>MNKVHVSAVGTGLLKNSLSADNVKKEVEDLGLKDWDRLKFDDDRQNKIRDNFTTLKDLLLNFLKSKGKEASAELDSLLSAIEKLQHKKEELYVFLYTTNTWNSKLAGEVIKNYLEEEGIKS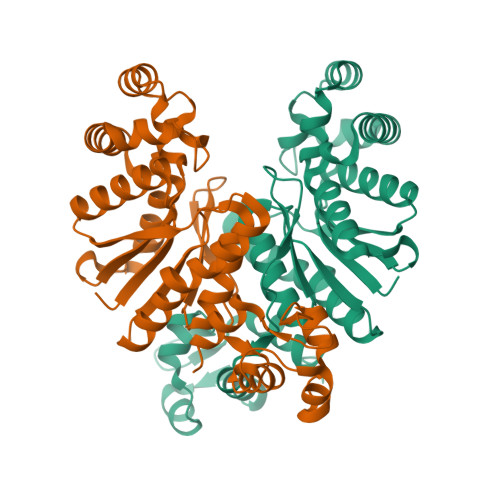ELATVKSISSEETFHEGIEDLFDKVIYKILKFKEEGKEVYINATAGLGPETTFLTLAGLLAGADLVYYKYQEFNDVVFLPSPPITISPRYLEWLIEFANYGYTLSEKKAEELGIPVRLLEVRNLVERKGEDAYRLKDWVRKMLGIYLGSEFELE[2x]> APEEERIKYVITVVEQIAKDAHRNGQEELAKLAERTAEEAKKATERGEEETLRIVYVIVVVLQIALEAHRNGQEELAKLALRTAEEAIKATERGEEETLRIVYVIVVVLQIALEAHRNGQEELAKLALRTAEEAIK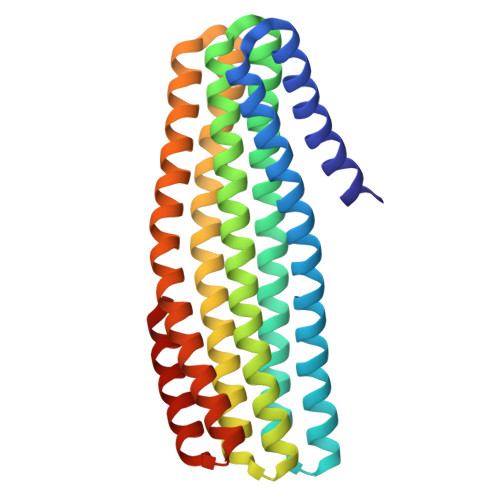ATERGEEETLRIVYVIVVVLQIALEAHRNGQEELAKLALRTAEEAIKATERGEEETLRIVYVIVVVLQIALEAHRNGQEELAKLALRTAEEAIKATERGEEETERIVYDIVVVLQEALEAHRNGEEERAKKALDEARRRIEATERGE> GAMQNNNEFKIGNRSVGYNHEPLIICEIGINHEGSLKTAFEMVDAAYNAGAEVVKHQTHIVEDEMSDEAKQVIPGNADVSIYEIMERCALNEEDEIKLKEYVESKGMIFISTPFSR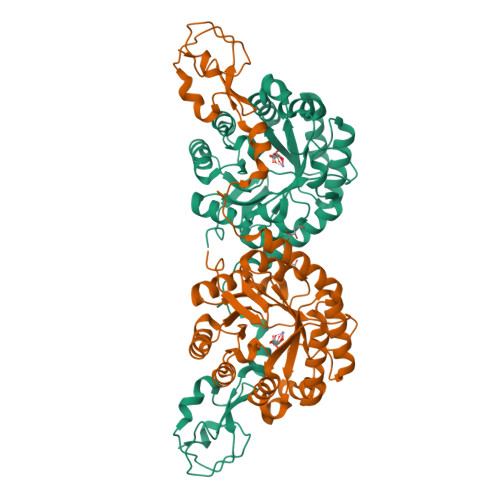AAALRLQRMDIPAYKIGSGECNNYPLIKLVASFGKPIILSTGMNSIESIKKSVEIIREAGVPYALLHCTNIYPTPYEDVRLGGMNDLSEAFPDAIIGLSDHTLDNYACLGAVALGGSILERHFTDRMDRPGPDIVCSMNPDTFKELKQGAHALKLARGGKKDTIIAGEKPTKDFAFASVVADKDIKKGELLSGDNLWVKAPGNGDFSVNEYETLFGKVAACNIRKGAQIKKTDIE>[2x]SPVAGHDAVSHEEKRQSTSFWYANMDHTGNARGFAPDLDGDFSYAVYKAVAPGDAAGIQRAINEGTGGVRRHGEWLASQPRVVYIPPGTYTISSTIFMNTDTILMGDATNPPVLKAAAGFSGNRILLDGRDPSITDGRGELSFAVGLKNLILDTTNIQGGQEFTALHWGVAQVAQLQNIKIRMSPSVSGSSTGHTGIRLTRGSTLALADVRLERGLNGIWHDGHQQALYKSIYFYQNTVGMLITNGATISILAPTFETVGTGVLCTSGAPYIGLVDARSINSGVTLKTTTYPSFLIENLNKDAQSSSNVAEGPSGTILNNRAHVDTFTYGNTVGRNPVYGDTYTTNTRPPALAPGGKYPVLPAPNYAANTVADFINVKDPAQNGGRTVLGDNTKDESKVLNEILQLAASTNKIAYFPFGKYRVDDTLLVPRGSRIVGEAWSTITGNGDKFKDESNPRPVVKVGNAGDVGVAQISDMRITISDVMPGAILIQFNMAGSNPGDVALWNSLITIGGTRGANALNSKCKDARNECKAAFLGMHFTTSSSAYVENVWNWVTDHGTEAYDSGSNIAAKGGALVESTRGTWLHALGSEHYWLYQLNLRKASNVMISLLQSETNYDQGDNVQQAPPAPWTPNVTGWGDPDFSWCGPNDTRCRMGFSNYINGGSNIYTYASASWAFFSGPGYQNCAGEFACQNHLHWIEQAPTNLQAFGICGKGSWAALRLAGGNVITSEPDFKGGWNGGGGGSLVGRYTP

The glycoside hydrolase family 55 (GH55) includes inverting exo-β-1,3-glucosidases and endo-β-1,3-glucanases, acting on laminarin, which is a β1-3/1-6-glucan consisting of a β1-3/1-6-linked main chain and β1-6-linked branches. Here, we investigated the mechanism of endo-type action on laminarin by GH55 endo-β-1,3-glucanase MnLam55A, identified from Microdochium nivale. MnLam55A was identified from extracellular proteins of a phytopathogenic fungus Microdochium nivale, which infects grasses and cereals and causes pink snow mold. NMR analysis of the initial degradation of laminarin revealed that MnLam55A preferentially cleaved the nonreducing terminal β1-3-linkage of the laminarioligosaccharide moiety at the reducing end side of the main chain β1-6-linkage.

The crystal structure of MnLam55A was determined in unliganded form at 2.4 Å resolution. The solved structure contains two molecules of MnLam55A in the asymmetric unit. The entire structure consists of two β-helical domains of 3-solenoid connected by a linker. Each of the domains is composed of 12 coils, which each contains three strands and three loops as observed in GH55 exo-β-1,3-glucosidases. In MnLam55A, the catalytic site and subsite −1 are formed by Glu-140, Gln-172, Ser-203, Trp-552, Asp-557, Glu-591, His-592, Glu-614, and Tyr-617, the aromatic block is formed by Phe-143, Trp-552, and Trp-554, and subsite +1 is formed by Gln-225, Tyr-617, Phe-677, and Phe-678. These residues are spatially conserved well with those of exo-β-1,3-glucosidases. As the plus subsites for the binding of longer oligosaccharides, the aromatic residues suggested in SacteLam55A (Trp-196 at subsite +2 and Tyr-194 at subsite +5) and those on the putative substrate binding groove in PcLam55A (Tyr-135, Phe-199, and Trp-245) are not observed in MnLam55A. On the contrary, MnLam55A has an open cleft, extending from subsite −2 toward the nonreducing part-binding site, to place 3-hydroxy group of the d-glucosyl residue in subsite −2 toward an open space on the cleft in the docking model. The cleft-forming residues of N-domain, Trp-75, Thr-135, and Leu-141 of MnLam55A, are conserved well in other endo-β-1,3-glucanase sequences, which suggests their importance for the formation of minus subsites. The smaller size of C5-L3 in the structure probably allows the localization of C6-L3 appropriately for the formation of the extended cleft and possible subsites.> MDNKITPADEEKIREWLNCEEASVDNDGDVWVAVPMTGHWLSDEQKAKYIEWRGDE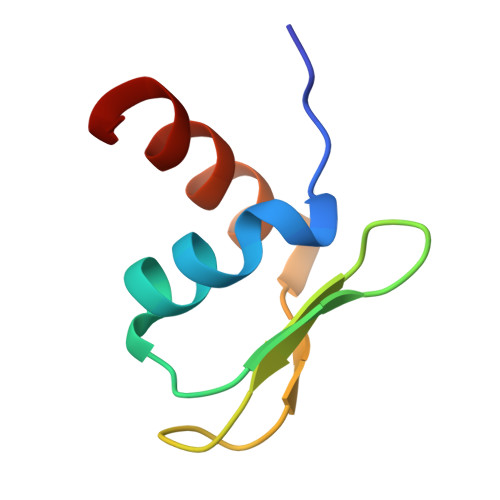T>MSKYKLIMLRHGEGAWNKENRFCSWVDQKLNSEGMEEARNCGKQLKALNFEFDLVFTSVLNRSIHTAWLILEELGQEWVPVESSWRLNERHYGALIGLNREQMALNHGEEQVRLWRRSYNVTPPPIEESHPYYQEIYNDRRYKVCDVPLDQLPRSESLKDVLERLLPYWNERIAPEVLRGKTILISAHGNSSRALLKHLEGISDEDIINITLPTGVPILLELDENLRAVGPHQFLGDQEAIQAAIKK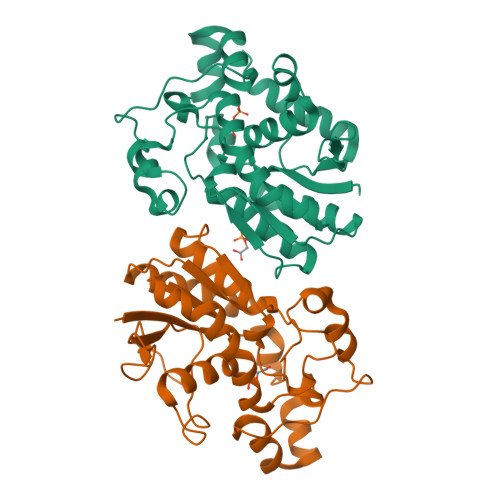VEDQGKVKQAKKLEHHHHHH[2x]> MKRQGKRPSKNLKARCSRKALHVNFKDMGWDDWIIAPLEYEAFHCEGLCEFPLRSHLEPTNHAVIQTLMNSMDPESTPPTCCVPTRLSPISILFIDSANN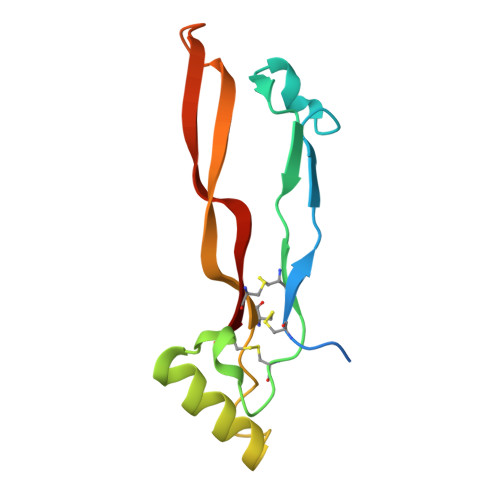VVYKQYEDMVVESCGCR2'-deoxy-1-methyl-pseudouridine | C10 H14 N2 O5 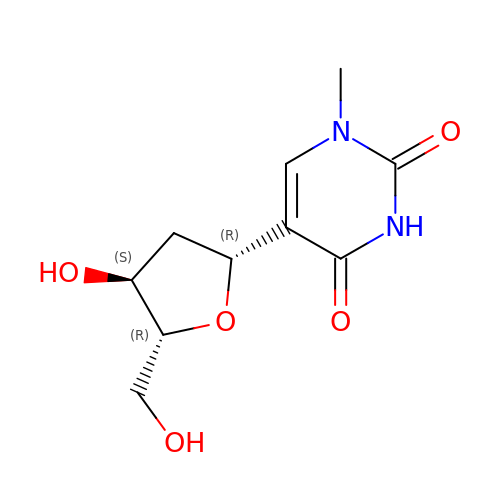| AMDJRICBYOAHBZ-XLPZGREQSA-N(1R,3S,5Z)-5-[(E)-3-[3,5-bis(6-methyl-6-oxidanyl-heptyl)phenyl]prop-2-enylidene]-4-methylidene-cyclohexane-1,3-diol | C32 H50 O4 | 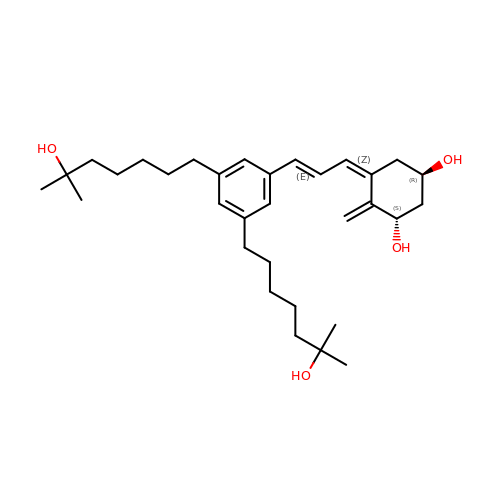KAXCFKOQLQAHBM-UHLYCMHWSA-N5-O-phosphono-alpha-D-ribofuranose | C5 H11 O8 P | 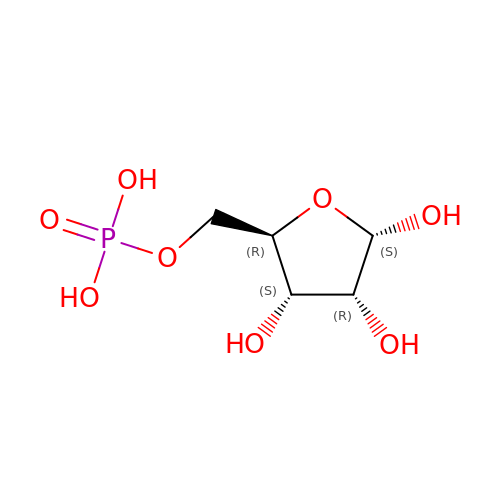KTVPXOYAKDPRHY-AIHAYLRMSA-N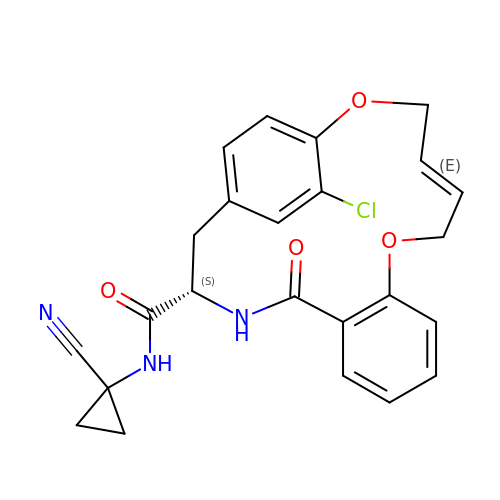(3~{S},14~{E})-19-chloranyl-~{N}-(1-cyanocyclopropyl)-5-oxidanylidene-12,17-dioxa-4-azatricyclo[16.2.2.0^{6,11}]docosa-1(21),6(11),7,9,14,18(22),19-heptaene-3-carboxamide | C24 H22 Cl N3 O4 | DAGMBGOOMHAGIF-RTLBZRNLSA-N>[2x]APQQINDIVHRTITPLIEQQKIPGMAVAVIYQGKPYYFTWGYADIAKKQPVTQQTLFELGSVSKTFTGVLGGDAIARGEIKLSDPTTKYWPEL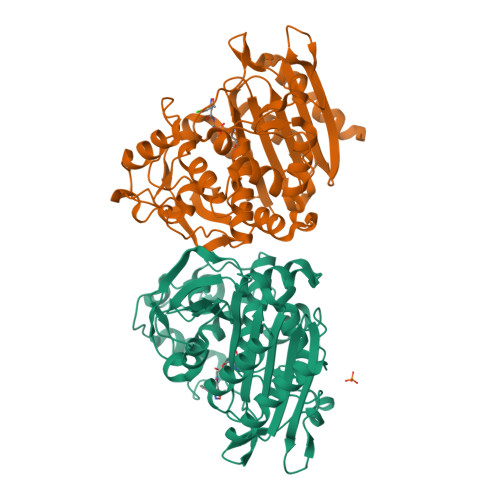TAKQWNGITLLHLATYTAGGLPLQVPDEVKSSSDLLRFYQNWQPAWAPGTQRLYANSSIGLFGALAVKPSGLSFEQAMQTRVFQPLKLNHTWINVPPAEEKNYAWGYREGKAVHVSPGALDAEAYGVKSTIEDMARWVQSNLKPLDINEKTLQQGIQLAQSRYWQTGDMYQGLGWEMLDWPVNPDSIINGSDNKIALAARPVKAITPPTPAVRASWVHKTGATGGFGSYVAFIPEKELGIVMLANKNYPNPARVDAAWQILNALA> PPVIRQGPVNQTVAVDGTFVLSCVATGSPVPTILWRKDGVLVSTQDSRIKQLENGVL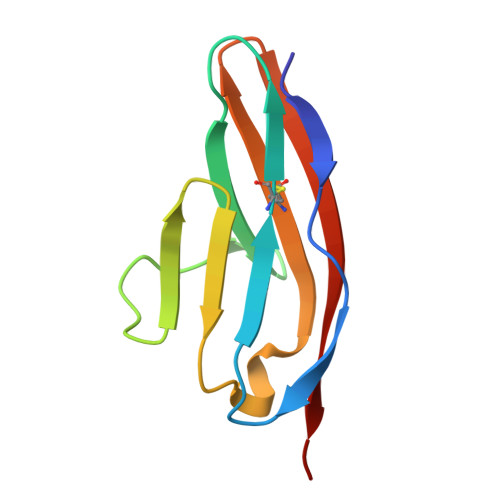QIRYAKLGDTGRYTCIASTPSGEATWSAYIEVQAG>[8x]HHHHHHHGHL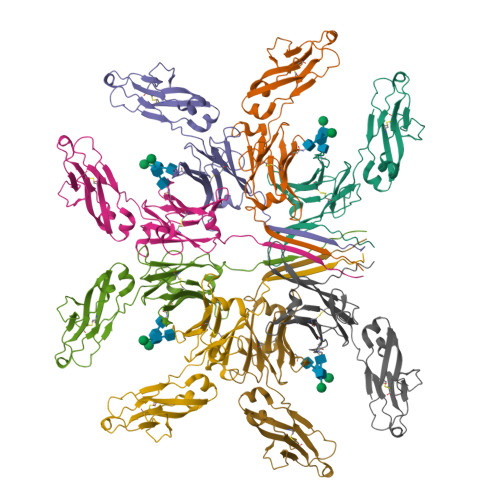VVITIIEPSLEDMLMNKKAQLVCDVNELVPGFLSVKWENDNGKTLTSRKGVTDKIAILDITYEDWSNGTVFYCAVDHMENLGDLVKKAYKRETGGVPQRPSVFLLAPAEQTSDNTVTLTCYVKDFYPKDVLVAWLVDDEPVERTSSSALYQFNTTSQIQSGRTYSVYSQLTFSNDLWKNEEVVYSCVVYHESMIKSTNIIMRTIDRTSNQPNLVNLSLNVPQRCMAQ Glycogen synthase (GYS1) is the central enzyme in muscle glycogen biosynthesis. GYS1 activity is inhibited by phosphorylation of its amino (N) and carboxyl (C) termini, which is relieved by allosteric activation of glucose-6-phosphate (Glc6P). We present cryo-EM structures at 3.0–4.0 Å resolution of phosphorylated human GYS1, in complex with a minimal interacting region of glycogenin, in the inhibited, activated and catalytically competent states. Each GYS1 monomer consisted of two Rossmann domains and a tetramerization domain and interacted with GYG1 in a 1:1 ratio.

While processing the GYS1–GYG1ΔCD + Glc6P data set, we observed that one three-dimensional (3D) class appeared similar to the inhibited (T) state and was refined to 4.0 Å resolution. Similar to our T state map, where phosphorylated Ser641 of the C terminus interacted with the arginine clusters, density for Glc6P in the allosteric site was apparent for this structure. Unlike the activated (R) state, Glc6P in this structure did not interact with subunits across the dimeric interface, because residues 290–292 remained disordered. In this ‘inhibited-like’ state, all interactions involved the phosphate group and were identical to the activated states except for Arg586, which was not in a productive conformation to interact with both glucose and phosphate moieties of Glc6P. However, 3D variability analysis of the Glc6P-bound inhibited-like state showed a unique movement not observed in the inhibited state without Glc6P. This appeared as a 2.0 Å expansion of the complex from the tetrameric interface; by flexibly fitting our inhibited-state model, we observed that helix α13 moved towards the regulatory helices. However, the R state is in a dynamic equilibrium with an inhibited-like state, owing to competition between the locking interactions of phosphorylated termini at the subunit interface and the conformational change due to Glc6P binding.

>MPLNRTLSMSSLPGLEDWEDEFDLENAVLFEVAWEVANKVGGIYTVLQTKAKVTGDEWGDNYFLVGPYTEQGVRTQVELLEAPTPALKRTLDSMNSKGCKVYFGRWLIEGGPLVVLLDVGASAWALERWKGELWDTCNIGVPWYDREANDAVLFGFLTTWFLGEFLAQSEEKPHVVAHFHEWLAGVGLCLCRARRLPVATIFTTHATLLGRYLCAGAVDFYNNLENFNVDKEAGERQIYHRYCMERAAAHCAHVFTTVSQITAIEAQHLLKRKPDIVTPNGLNVKKFSAMHEFQNLHAQSKARIQEFVRGHFYGHLDFNLDKTLYFFIAGRYEFSNKGADVFLEALARLNYLLRVNGSEQTVVAFFIMPARTNNFNVETLKGQAVRKQLWDTANTVKEKFGRKLYESLLVGSLPDMNKMLDKEDFTMMKRAIFATQRQSFPPVCTHNMLDDSSDPILTTIRRIGLFNSSADRVKVIFHPEFLSSTSPLLPVDYEEFVRGCHLGVFPSYYEPWGYTPAECTVMGIPSISTNLSGFGCFMEEHIADPSAYGIYILDRRFRSLDDSCSQLTSFLYSFCQQSRRQRIIQRNRTERLSDLLDWKYLGRYYMSARHMALSKAFPEHFTYEPNEADAAQGYRYPRPASVPPSPSLSRHSSPHQSEDEEDPRNGPLEEDGERYDEDEEAAKDRRNIRAPEWPRRASCTSSTSGSKRNSVDTATSSSLSTPSEPLSPTSSLGEERN[4x];>MTDQAFVTLTTNDAYAKGALVLGSSLKQHRTTRRLVVLATPQVSDSMRKVLETVFDEVIMVDVLDSGDSAHLTLMKRPELGVTLTKLHCWSLTQYSKCVFMDADTLVLANIDDLFDREELSAAPDPGWPDCFNSGVFVYQPSVETYNQLLHLASEQGSFDGGDQGILNTFFSSWATTDIRKHLPFIYNLSSISIYSYLPAFKVFGASAKVVHFLGRVKPWNYTYDPKTKSVKSEAHDPNMTHPEFLILWWNIFTTNVLPLLQQFGLVKDTCSYVNVLSDLVYTLAFSCGFCRKEDVSGAISHLSLGEIPAMAQPFVSSEERKERWEQGQADYMGADSFDNIKRKLDTYLQ[4x]>[2x]MDNREIVMKYISYKLSQRGYEW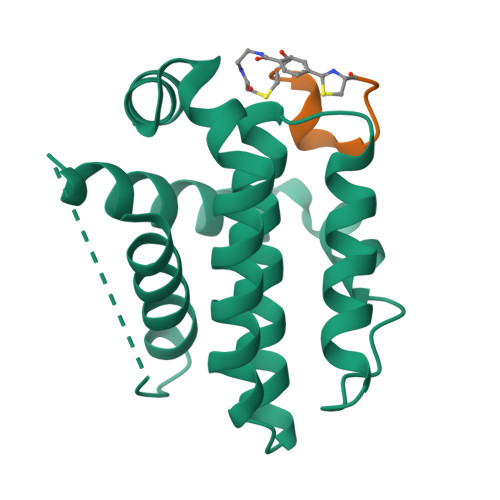DAGDVEENRTEAPEGTESEVVHQTLRQAGDDFSLRYRRDFAEMSSQLHLTPGTAYASFATVVEELFRDGVNWGRIVAFFEFGGVMCVESVNREMSVLVDNIAAWMATYLNDHLHTWIQDNGGWDAFVELYG;>[2x]APIRYEWDEFC> NQLAWF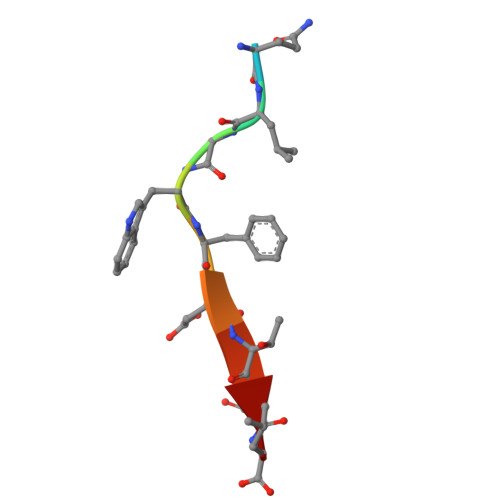DTDL>[2x]VGSADAPAPYRV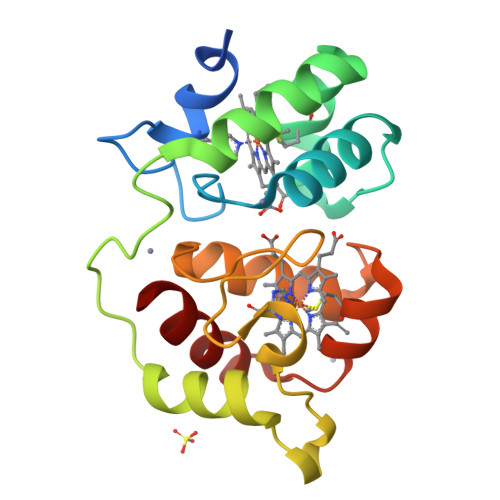SSDCMVCHGMTGRDTLYPIVPRLAGQHKSYMEAQLKAYKDHSRADQNGEIYMWPVAQALDSAKITALADYFNAQKPPMQSSGIKHAGAKEGKAIFNQGVTNEQIPACMECHGSDGQGAGPFPRLAGQRYGYIIQQLTYFHNGTRVNTLMNQIAKNITVAQMKDVAAYLSSL>[2x]PPYTIVYFPVRGRCEAMRMLLADQGQSWKEEVVTIDTWMQGLLKPTCLYGQLPKFEDGDLTLYQSNAI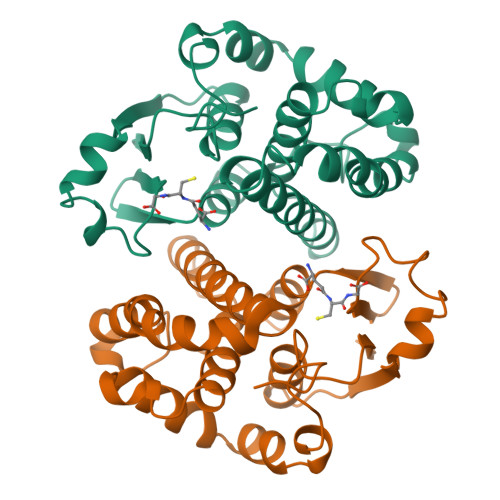LRHLGRSLGLYGKNQREAAQMDMVNDGVEDLRGKYVTLIYTNYENGKNDYVKALPGHLKPFETLLSQNQGGKAFIVGDQISFADYNLLDLLLIHQVLAPGCLDNFPLLSAYVARLSARPKIKAFLSSPEHVNRPINGNGKQ>SVSIQAFTLEYIEVATERYKTLIGEGGFGSVYRGTLNDGQEVAVKVRSATSTQGTREFDNELNLLSAIQHENLVPLLGYCNESDQQILVYPFMSNGSLQDRLYGEPAKRKILDWPTRLSIALGAARGLAYLHTFPGRSVIHRDIKSSNILLDHSMCAKVANFGFSKYAPQEGDSYVSLEVRGTAGYLDPEYYKTQQLSEKSDVFSFGVVLLEIVSGREPLNIKRPRTEWSLVEWATPYIRGSKVDEIVDPGIKGGYHAEAMWRVVEVALQCLEPFSTYRPSMVAIVRELEDALIIENNAS[3x]

Symbiosis between legumes and nitrogen-fixing bacteria is dependent on the Symbiosis receptor-like kinase (SYMRK). Nod factors produced by rhizobia are recognized by the LysM receptors NFR1 and NFR5 (2–5) in Lotus japonicus (Lotus), and these receptors subsequently transduce the signal to the malectin-like/leucine-rich repeat receptor kinase SYMRK. SYMRK is the first component of the common symbiotic pathway driving symbiosis with rhizobia, Frankia, and arbuscular mycorrhizal fungi. The SYMRK receptor has an active intracellular kinase domain, and mutations in the core kinase domain have been linked to loss of symbiotic function, showing that kinase activity is important for root nodule formation.

To understand the signaling function of SYMRK in root nodule symbiosis, we expressed, purified, and determined the crystal structure of the core kinase domain. A diffraction dataset extending to 1.95 Å was collected, and the phase problem was solved by molecular replacement using a homology model created from the Arabidopsis thaliana BIK1 kinase structure. The overall crystal structure of the SYMRK kinase domain resembles other eukaryotic kinases of the IRAK4/Pelle-type and A. thaliana BAK1 (16) and BIK1. As predicted from the sequence, SYMRK has all the canonical structural motifs required for ATP binding and catalytic activity. The SYMRK kinase crystallized in an inactive conformation, with a broken catalytic spine (C-spine) due to the lack of a bound nucleotide. However, ATP can easily be docked into its predicted binding site. The regulatory spine (R-spine) is assembled, but the C-helix is in an inactive “out” position, leaving the salt bridge between the catalytic lysine (K622) and αC-glutamate (E638) broken. We mapped the phosphorylation sites onto the structure of SYMRK and used Alphafold2 to model the remaining C-terminal part missing in the crystal structure. The phosphorylation sites are located in three distinct regions, with five in the kinase core domain (S731, S751, S754, T760, and S807), four sites in the border region between the kinase domain and the distal C-terminal tail, which we named the “alpha-I motif” (S877, S885, S889, and S893), and seven sites in the distal C-terminal tail region (S903, T905, S906, S910, T911, S916, and S918). The mechanism of SYMRK activation is possibly trans-autophosphorylation since the alpha-I motif is located within an extended alpha-I helix that sterically would hinder cis-autophosphorylation.> MWPPRLLSCIFTIILIVAVIAPTSDSTTVRRRLRKPSKSVSVTSSVSRSTDQVISASVNRPKIRGRPSVASRKSSAALDNSVGTDDHKDKDGYKIV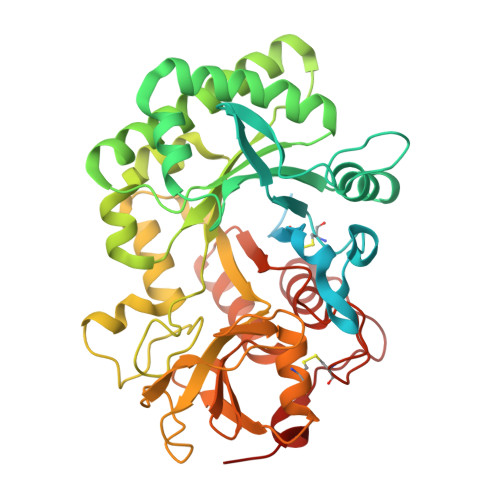CYYTNWSQYRTKIGKFMPEDIQPELCTHIIFAFGWLKKGKLSSFESNDETKDGKTGLYDRINALKKANPKLKTLLAIGGWSFGTQKFKEMSATRYARQTFIYSAIPYLRDRNFDGLDIDWEYPKGGDDKKNYVLLLKELREAFEAEAQEVKKPRLLLTAAVPVGPDNIKSGYDVPAVASYLDFINLMAYDFHGKWERETGHNAPLYAPSSDSEWRKQLSVDHAAHLWVKLGAPKEKLIIGMPTYGRTFTLSNPNNFKVNSPASGGGKAGEYTKESGFLAYYEVCEILRNGGAYVWDDEMKVPYAIHGDQWVGFDDEKSIRNKMRWIKDNSFGGAMVWTVDMDDFSGGVCGGNVKYPLIGAMREELRGISRGKDAKDVDWASVAASV> MKAKRVQAKI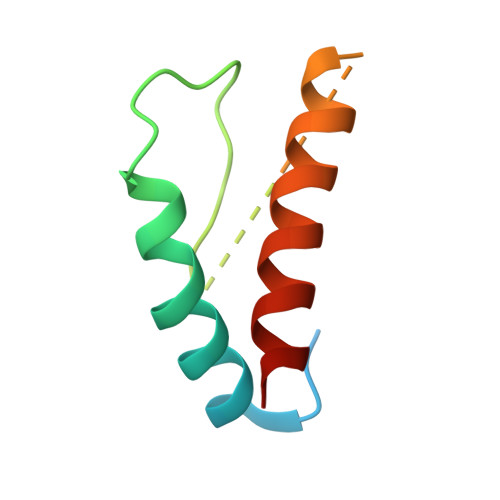EIEFPSEDVAKVVYEAVLYEHLSVPYRRSEIDFKLEGKKIILDIKATDSSALRGTVNSYLRWIKAAIDVIEV> AEQKTLHIYNWTDYIAPDTVANFEKETGIKVVYDVFDSNEVLEGKLMAGSTGFDLVVPSASYLERQLTAGVFQPLDKSKLPEWKNLDPELLKLVAKHDPDNKFAMPYMWATTGIGYNVDKVKAVLGENAPVD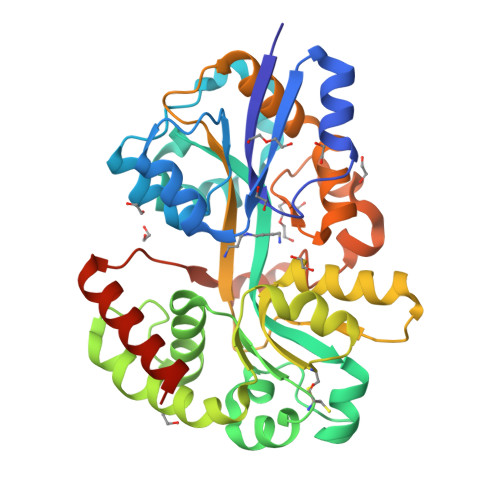SWDLILKPENLEKLKSCGVSFLDDPEEVFATVLNYLGKDPNSTKADDYTGPATDLLLKLRPNIRYFHSSQYINDLANGDICVAIGWAGSVWQASNRAKEAKNGVNVSFSIPKEGAMAWFDVFAMPADAKNKDEAYQFLNYLLRPDVVAHISDHVFYANANKAATPLVSAEVRENPGIYPPADVRAKLFTQKVQDPKIDRVRTRAWTKVKSGKLEHHHHHH> QTQQEEEEEDEDHGPDDYDEEDEDEVEEEETNRLPGGRSRVLLRCYTCKSLPRDERCDLTQDCSHGQTCTTLIAHGNTESGLLTTHSTWCTDSCQPITKTVEGTQVTMTCCQSSLCNVP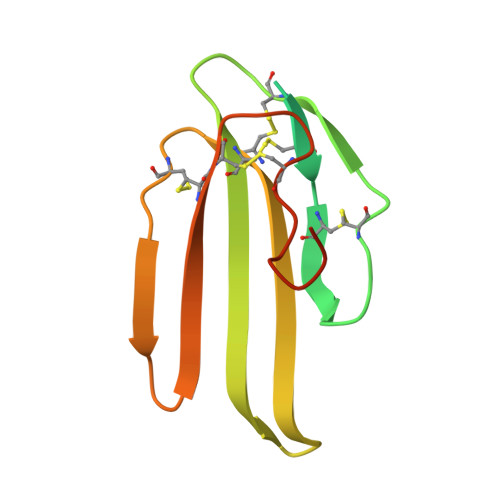PWQSSRVQDPTG> GSPLRKFKLVFLGEQSVGKTSLITRFMYDSFDNTYQATIGIDFLSKTMYLEDRTIRLQLWDTAGQERFRSLIPSYIRDSAAAVVVY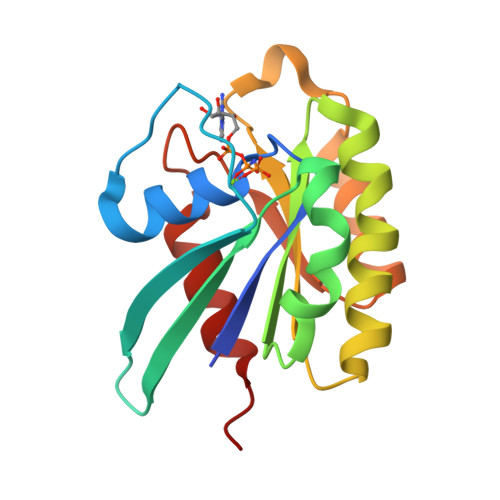DITNVNSFQQTTKWIDDVRTERGSDVIIMLVGNKTDLADKRQVSIEEGERKAKELNVMFIETSAKAGYNVKQLFRRVAAALPGM> MPREFKS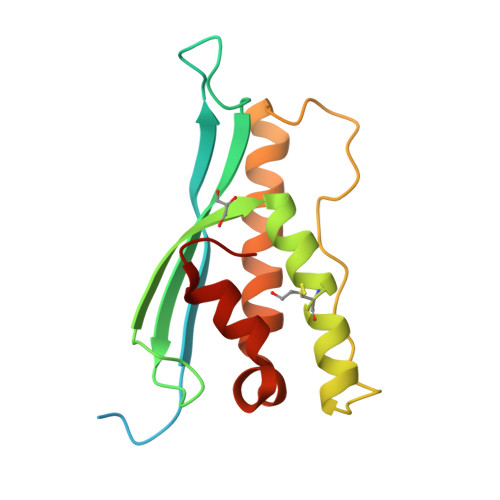FGSTEKSLLSKGHGEPSYSEIYAEPENFLEIEVHNPKTHIPNGMDSKGMFTDYEIICRTNLPSFHKRVSKVRRRYSDFEFFRKCLIKEISMLNHPKVMVPHLPGKILLSNRFSNEVIEERRQGLNTWMQSVAGHPLLQSGSKVLVRFIEAEKFVG5-NITROINDAZOLE | C7 H5 N3 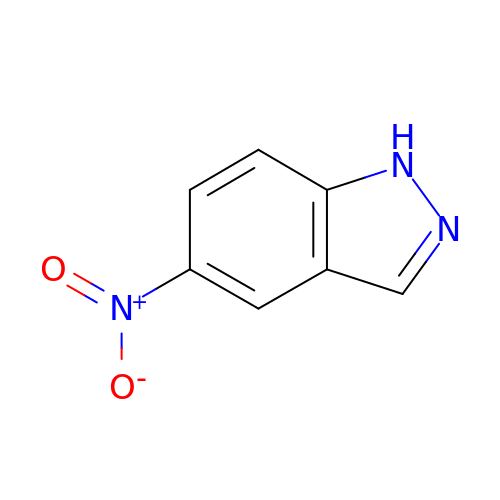O2 | WSGURAYTCUVDQL-UHFFFAOYSA-N>[4x]MALTTTGTEQHDLFSGTFWQNPHPAYAALRAEDPVRKLALPDGPVWLLTRYADVREAFVDPRLSKD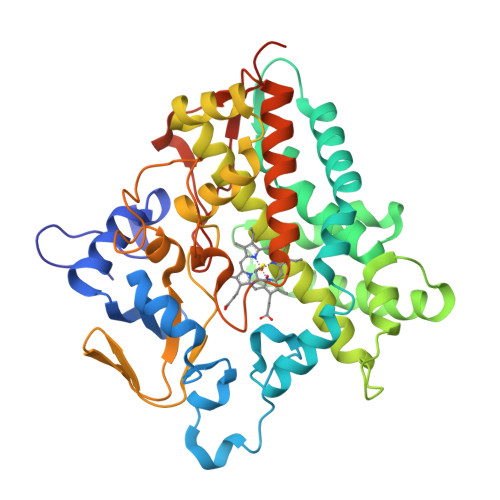WRHTLPEDQRADMPATPTPMMILMDPPDHTRLRKLVGRSFTVRRMNELEPRITEIADGLLAGLPTDGPVDLMREYAFQIPVQVICELLGVPAEDRDDFSAWSSVLVDDSPADDKNAAMGKLHGYLSDLLERKRTEPDDALLSSLLAVSDEDGDRLSQEELVAMAMLLLIAGHETTVNLIGNGVLALLTHPDQRKLLAEDPSLISSAVEEFLRFDSPVSQAPIRFTAEDVTYSGVTIPAGEMVMLGLAAANRDADWMPEPDRLDITRDASGGVFFGHGIHFCMGAQLARLEGRVAIGRLFADRPELALAVGLDELVYRESTLVRGLSRMPVTMGPRSALEHHHHHH2-methoxy-4-[4-methyl-5-(4-piperazin-1-ylphenyl)pyridin-3-yl]benzamide | 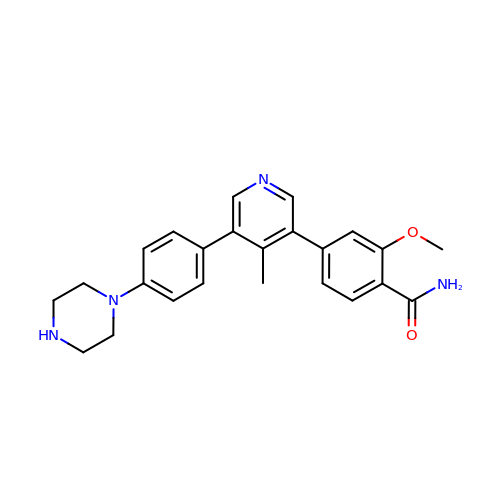C24 H26 N4 O2 | GFEAXKZXFORDDU-UHFFFAOYSA-N> MWRLSRSLRSNSLHNPGPFLDGALQLIKL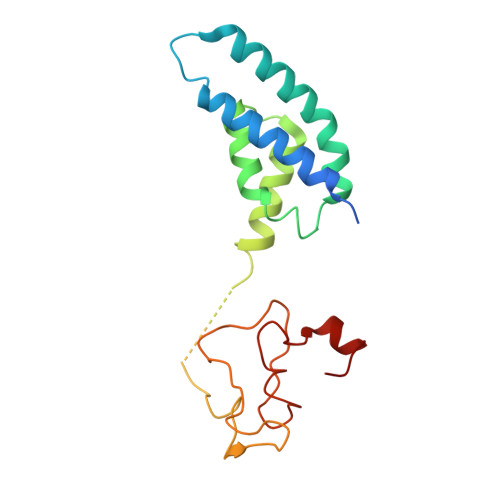HLAHKNAAADKNTKACSDIEGEFLRELEAFRACFTMSSSLKVAKLYTKKLHGALSYFQLYDDPLMRQLDMIIGKQTMQPSAGRQHGVFKAPVAARLDPFFLDEREETVLPSELPNPPKPDPSTPLRERALKVPAQHRGHWVLRDPDIAITREERRTDPW> MEEIYAKFVSQKISKTRWRPLPPGSLQTAETFATGSWDNEENYISLWSIGDFGNLDSDGGFEGDHQLLCDIRHHGDVMDLQFFDQERIVAASSTGCVTVFLHHPNNQTLSVNQQWTTAHYHTGPGSPSYSSAPCTGVVCNNPEIVTVGEDGRINLFRADHKEAVRTIDNADSSTLHAVTFLRTPEILTVNSIGQLKIWDFRQQGNEPSQ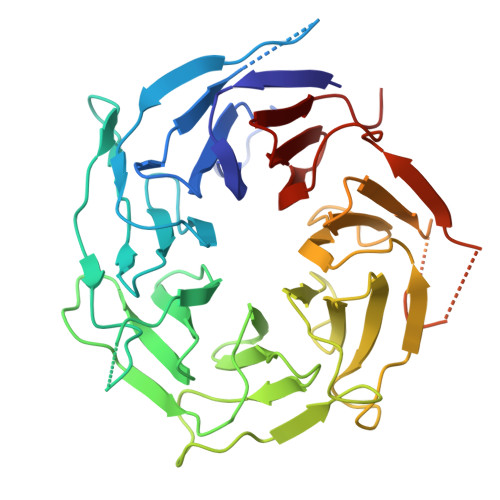ILSLTGDRVPLHCVDRHPNQQHVVATGGQDGMLSIWDVRQGTMPVSLLKAHEAEMWEVHFHPSNPEHLFTCSEDGSLWHWDASTDVPEKSSLFHQGGRSSTFLSHSISNQANVHQSVISSWLSTDPAKDRIEITSLLPSRSLSVNTLDVLGPCLVCGTDAEAIYVTRHLFS>ADKELKFLVVDDFSTMRRIVRNLLKELGFNNVEEAEDGVDALNKLQAGGYGFVISDWNMPNMDGLELLKTIRADGAMSALPVLMVTAEAKKENIIAAAQAGASGYVVKPFTAATLEEKLNKIFEKLGM[2x];>[2x]RQLALEAKGETPSAVTRLSVVAKSEPQDEQSRSQSARRIILSRLKAGEVDLLEEELGHLTTLTDVVKG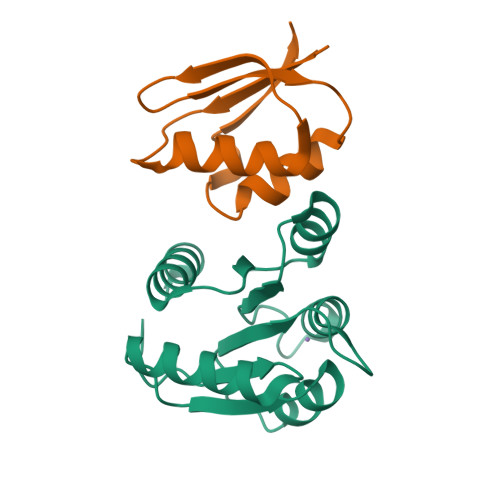ADSLSAILPGDIAEDDITAVLCFVIEADQITFETVEVSPKISTPPVLKLAAEQAPTGRVEREKTTR>GMSLIEIRKRTLIVETTYHENGPAPAQPLKLAASCAVIRNPYAGRYEPDLMPFMAELRSLGTLLATELVDTLGKDNIEVYSKAA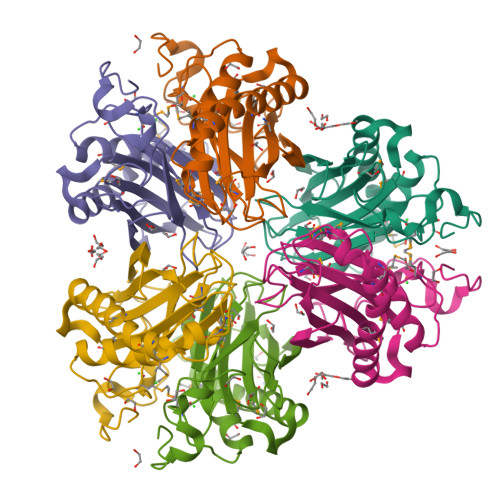IVGVDGEMEHGAVWHEAGGWAMRSVLGEPKAMVPAVKAVATAGYRMMVPVHYIHASYVRSHFNSIEIGIQDAPRPREILFALVMGTGARVHARLGGLTKEAVSVHDGQR[3x]>MEFTTGLMSLDTALNEMLSRVTPLTAQETLPLVQCFGRILASDVVSPLDVPGFDNSAMDGYAVRLADIASGQPLPVAGKSFAGQPYHGEWPAGTCIRIMTGAPVPEGCEAVVMQEQTEQMDNGVRFTAEVRSGQNIRRRGEDISAGAVVFPAGTRLTTAELPVIASLGIAEVPVIRKVRVALFSTGDELQLPGQPLGDGQIYDTNRLAVHLMLEQLGCEVINLGIIRDDPHALRAAFIEADSQADVVISSGGVSVGEADYTKTILEELGEIAFWKLAIKPGKPFAFGKLSNSWFC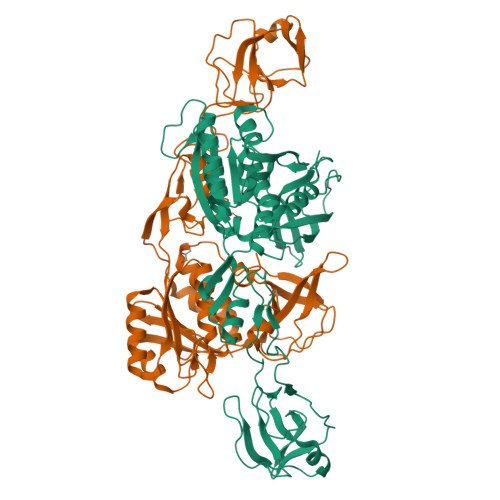GLPGNPVSATLTFYQLVQPLLAKLSGNTASGLPARQRVRTASRLKKTPGRLDFQAGVLQRNADGELEVTTTGHQGSHIFSSFSLGNCFIVLERDRGNVEVGEWVEVEPFNALFGGL[2x]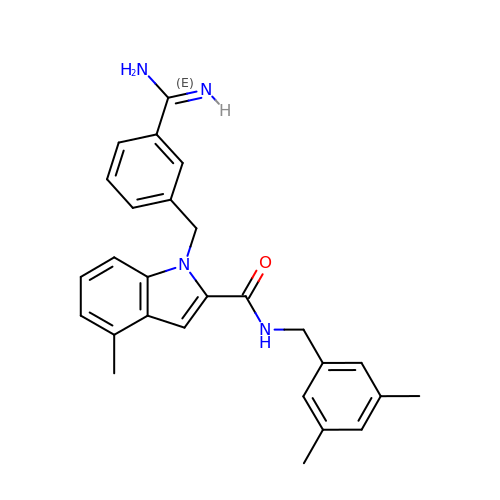1-(3-CARBAMIMIDOYL-BENZYL)-4-METHYL-1H-INDOLE-2-CARBOXYLIC ACID 3,5-DIMETHYL-BENZYLAMIDE | C27 H28 N4 O | JSQZLEYFOOSZPU-UHFFFAOYSA-N methyl 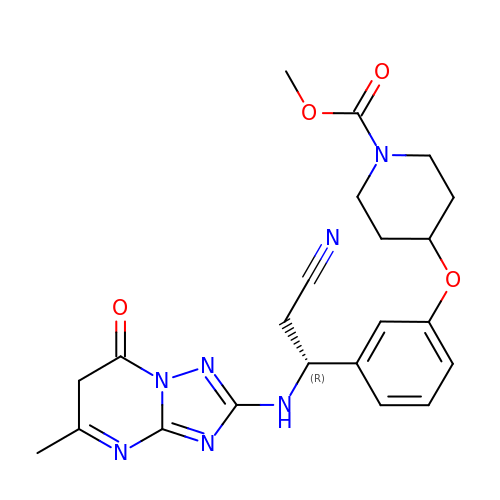4-(3-{(1R)-2-cyano-1-[(5-methyl-7-oxo-6,7-dihydro[1,2,4]triazolo[1,5-a]pyrimidin-2-yl)amino]ethyl}phenoxy)piperidine-1-carboxylate | C22 H25 N7 O4 | BAVCOKCQUYWPLU-GOSISDBHSA-N> LKESPSGYLRSGEGDTGCGELVWVGEPLTLRTAETITGKYGVWMRDPKPTYPYTQETTWRIDTVGTDVRQVFEYDLISQFMQGYPSKVHILPRPLESTGAVVYSGSLYFQGAESRTVIRYELNTKTVKAEKEIPGAGYHGQFPYSWGGYTDIDLAVDEAGLWVIYSTDEAKGAIVLSKLNPENLELEQTWETNIRKQSVANAFIICGTLYTVSSYTSADATVNFAYDTGTGISKTLTIPFKNRYKYSSMIDYNPLEKKLFAWDNLNMVTYD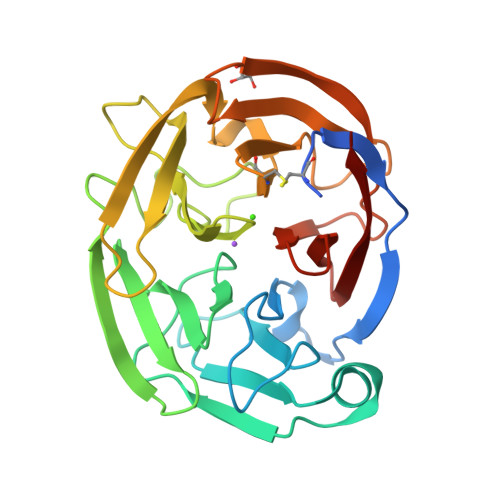IKLSKM> AQHITPVSEKKVDDKITLYKTTATSDNDKLNISQILTFNFIKDKSYDKDTLVLKAAGNINSGYKKPNPKDYNYSQFYWGGKYNVSVSSESNDAVNVVDYAPKNQNE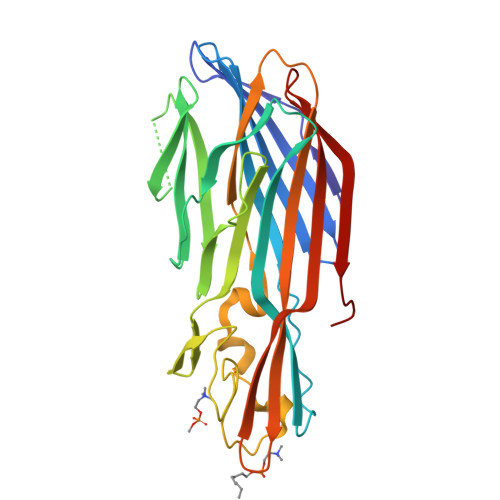EFQVQQTLGYSYGGDINISNGLSGGLNGSKSFSETINYKQESYRTTIDRKTNHKSIGWGVEAHKIMNNGWGPYGRDSYDPTYGNELFLGGRQSSSNAGQNFLPTHQMPLLARGNFNPEFISVLSHKQNDTKKSKIKVTYQREMDRYTNQWNRLHWVGNNYKNQNTVTFTSTYEVDWQNHTVKLIGTDSKETNPGV> AALENPGTVEELHKKCKDIQAITFEGAKIMLNKGLSNHFQVSHTINMSNVVPSGYRFGATYVGTKEFSPTEAFPVLLGDIDPAGNLNANVIHQFSARLRCKFASQIQESKVVASQLTTDYRGSDYTLSLTVANPSIFTNSG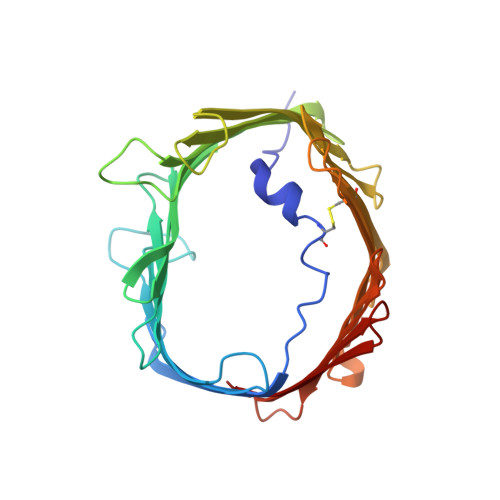VVVGQYLQSVTPALALGSELAYQFGPNVPGRQIAIMSVVGRYTAGSSVWSGTLGQSGLHVCYYQKASDQLQIGAEVETSLRMQESVATLAYQIDLPKANLVFRGGIDSNWQIFGVLEKRLAPLPFTLALSGRMNHVKNNFRLGCGLMIG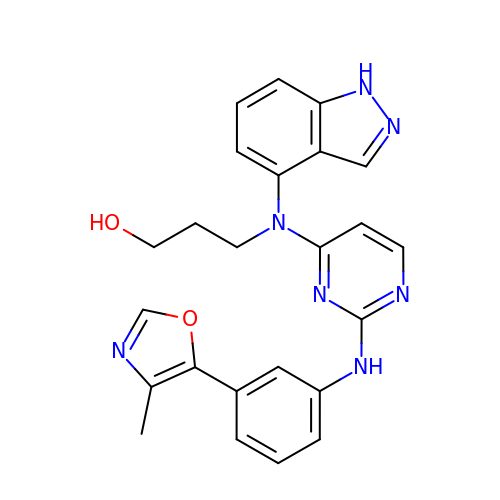3-[1H-indazol-4-yl(2-{[3-(4-methyl-1,3-oxazol-5-yl)phenyl]amino}pyrimidin-4-yl)amino]propan-1-ol | C24 H23 N7 O2 | ONJMWLWJHWIOQJ-UHFFFAOYSA-N>[2x]MSGTEDERRELEKVARKAIEAAREGNTDEVREQLQRALEIARESGSEEAFKLALEVVRRVAEVAARAGNVEAVK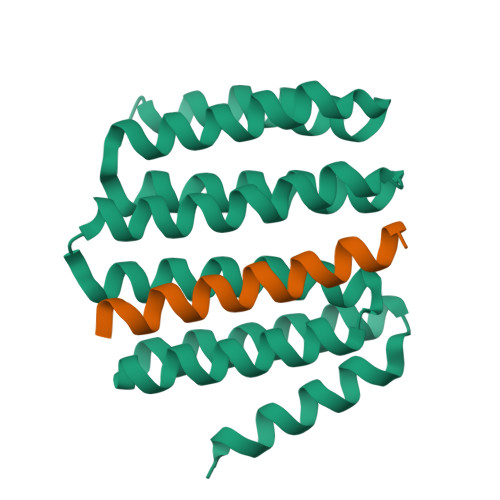EALRVALEIVKEAMELIKDPEAIVRLALEAVRVVAEVAARAGAVEAVKVALRVALEIAKIAGTEEAVRLALEVVKRVSDIAKKAGNEDAVKEAEEVRKKIEEESGGSGMEEARKELTREMIEVLREIEEGFKERFE Citrate synthase (CS) plays a central metabolic role in aerobes and many other organisms. The CS reaction comprises two half-reactions: a Claisen aldol condensation of acetyl-CoA (AcCoA) and oxaloacetate (OAA) that forms citryl-CoA (CitCoA), and CitCoA hydrolysis. Protein conformational changes that ‘close’ the active site play an important role in the assembly of a catalytically competent condensation active site. CS from the thermoacidophile Thermoplasma acidophilum (TpCS) possesses an endogenous Trp fluorophore that can be used to monitor the condensation reaction.

The 2.2 Å resolution crystal structure of TpCS fused to a C-terminal hexahistidine tag (TpCSH6) reported here is an ‘open’ structure that, when compared with several liganded TpCS structures, helps to define a complete path for active-site closure. Positive difference electron density was observed early in refinement at two locations: a helix near the CD dimer interface and the nearby subunit D active site. A second sharp turn near residue His222D directs the tag sequence into the active site of subunit D, ending with a bidentate salt bridge formed between the C-terminal carboxylate of the tag residue His399A and the Arg271D guanidinium. The C-terminal residue His399 makes a side-chain contact with His222, a residue that provides a hydrogen bond (involving Nδ1) that polarizes the AcCoA enolate, and the terminal carboxylate contacts both His262 and Arg271, which bind carbonyl and α-carboxylate O atoms in OAA. His397 N∊2 forms a hydrogen bond to one carboxylate O atom in the critical active-site base Asp317, which is not directly contacted by either substrate. Two well ordered bicarbonate ligands were included in the final model. The striking finding that all four subunits adopt open conformations suggests that the TpCS dimer cannot close just one active site.

>[4x]PETEEISKGLEDVNIKWTRLTTIDGNKGILRYGGYSVEDIIASGAQDEEIQYLFLYGNLPTEQELRKYKETVQKGYKIPDFVINAIRQLPRESDAVAMQMAAVAAMAASETKFKWNKDTDRDVAAEMIGRMSAITVNVYRHIMNMPAELPKPSDSYAESFLNAAFGRKATKEEIDAMNTALILYTDHEVPASTTAGLVAVSTLSDMYSGITAALAALKGPLHGGAAEAAIAQFDEIKDPAMVEKWFNDNIINGKKRLMGFGHRVYKTYDPRAKIFKGIAEKLSSKKPEVHKVYEIATKLEDFGIKAFGSKGIYPNTDYFSGIVYMSIGFPLRNNIYTALFALSRVTGWQAHFIEYVEEQQRLIRPRAVYVGPAERKYVPIAERKVDKLAAALEHHHHHH>MEFTYSYLFRMISHEMKQKADQKLEQLDITNEQGHTLGYLYAHQQDGLTQNDIAKALQR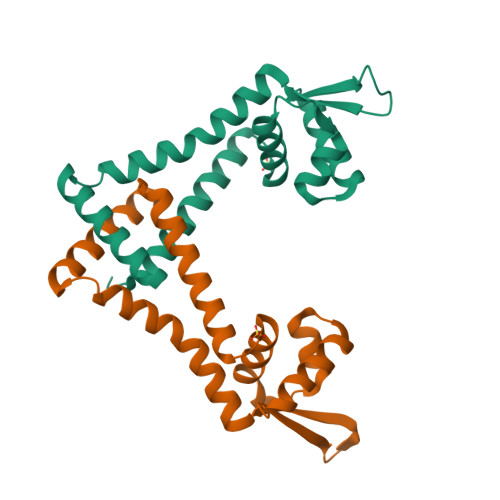TGPTVSNLLRNLERKKLIYRYVDAQDTRRKNIGLTTSGIKLVEAFTSIFDEMEQTLVSQLSEEENEQMKANLTKMLSSLQHHHHHH[2x]> EIHMTEFLDKLDFYVLPVVNIDGYIYTWTTNRMWRKTRSTRAGSSCTGTDLNRNFDAGWCSIGASNNPCSETYCGSAAESEKESKAVADFIRNHLSSIKAYLTIHSYSQMMLYPYSYDYKLPKNNVELNTLAKGAVKKLASLHGTTYSYGPGATTIYPASGGSDDWAYDQGIKYSFTFELRDKGRYGFVLPESQIQPTCEETMLAIKY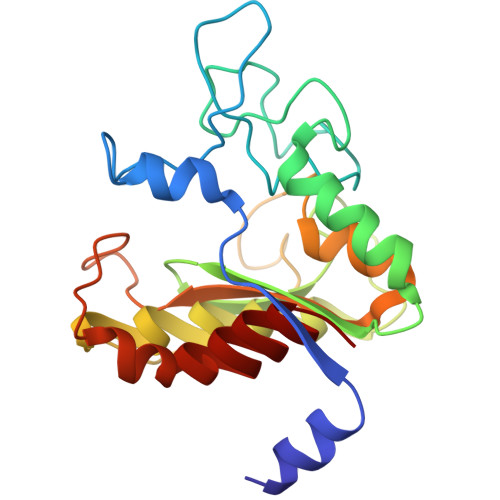VTSYVLEHL> MDSSTWSPKTTAVTRPVETHELIRNAADISIIVIYFVVVMAVGLWAMFSTNRGTVGGFFLAGRSMVWWPIGASLFASNIGSGHFVGLAGTGAASGIAIGGFEWNALVLVVVLGWLFVPIYIKAGVVTMPEYLRKRFGGQRIQVYLSLLSLLLYIFTKISADIFSGAIFINLALGLNLYLAIFLLLAITALYTITGGLAAVIYTDTLQTVIMLVGSLILTGFAFHEVGGYDAFMEKYMKAIPTIVSDGNTTFQEKCYTPRADSFHIFRDPLTGDLPWPGFIFGMSILTLWYWCTDQVIVQRCLSAKNMSHVKGGCILCGYLKLMPMFIMVMPGMISRILYTEKIACVVPSECEKYCGTKVGCTNIAYPTLVVELMPNGLRGLMLSVMLASLMSSLTSIFNSASTLFTMDIYAKVRKRASEKELMIAGRLFILVLIGISIAWVPIVQSAQSGQLFDYIQSITSYLGPPIAAVFLLAIFWKRVNEPGAFWGLILGLLIGISRMITEFAYGTGSCMEPSNCPTIICGVHYLYFAIILFAISFIT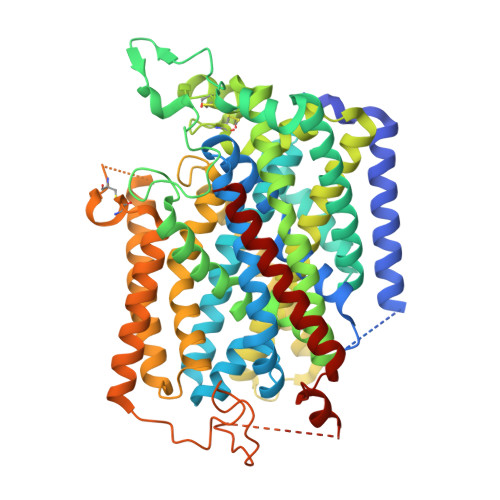IVVISLLTKPIPDVHLYRLCWSLRNSKEERIDLDAEEENIQEGPKETIEIETQVPEKKKGIFRRAYDLFCGLEQHGAPKMTEEEEKAMKMKMTDTSEKPLWRTVLNVNGIILVTVAVFCHAYFA> DAAQPARRARRTYEAYPAKPKC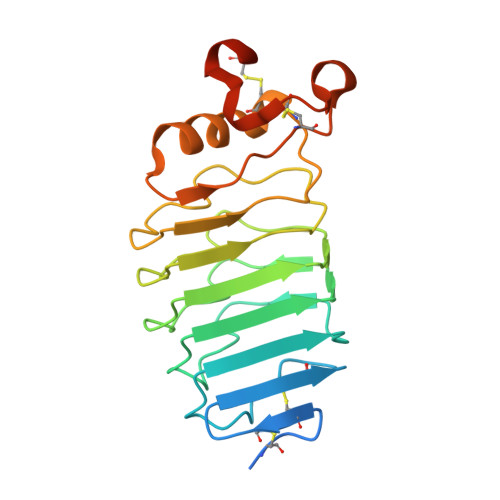PAVCTCTKDNALCENARSIPRTVPPDVISLSFVRSGFTEISEGSFLFTPSLQLLLFTSNSFDVISDDAFIGLPHLEYLFIENNNIKSISRHTFRGLKSLIHLSLANNNLQTLPKDIFKGLDSLTNVDLRGNSFNCDCKLKWLVEWLGHTNATVEDIYCEGPPEYKKRKINSLSSKDFDCIIKHHHHHH> MKLLHERMMHSLARYPRQTAVVDEQDALSYEALELRIREFVAMLCALGVGQGQRILLWAHKSVDLVAVMQAALRLGVVYVPVDPLSPVSRLEKIAGDSQAVLVLCTAARLEELAGSALAQVRSVVLDDPASAGYWRNIDTGSSVVPTLAIQPDDLAYILYTSGSTGVPKGVALSHGNALAFVDWACERYCFQPGERFANHAPLHFDLSVLDIYCALNVGATVCLVPESIAFSPRL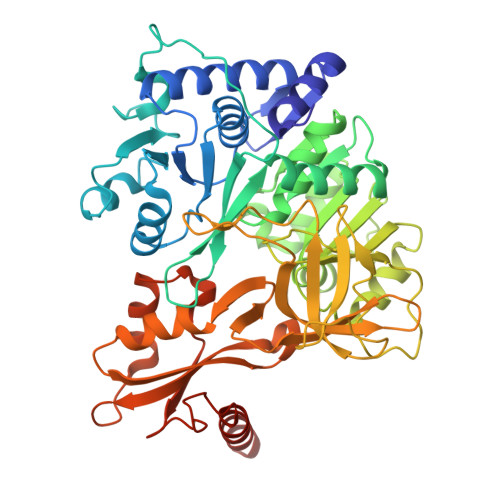LTDFIRQHEISIWYSVPSVLMMMMQDGDLLSDIQDTLRVLLFAGEPFPVKHLRDLRAAYADVRLANLFGPTETNVCTAFEVGAIDPERVLPVPIGTAASGNQVWAQKPDGSRCAVGEEGELVVQGPTVMLGYFAKPAQEGPYKTGDMVRQRPDGNYEYLGRRDDMLKVRGNRIERGEVEAALLAHPQVSEAAVLVVGEGMNAQLWGVLVAHTRDALSLIDLKRHCAQRLPRYMIIDKVLCLDALPRNANGKVDRFALARQVEGKLAAALEHHHHHHHH4-({(2S)-2-[2-(4-chlorophenyl)-5,6-difluoro-1H-benzimidazol-1-yl]-2-cyclohexylacetyl}amino)-3,5-difluorobenzoic acid | C28 H22 Cl F4 N3 O3 | 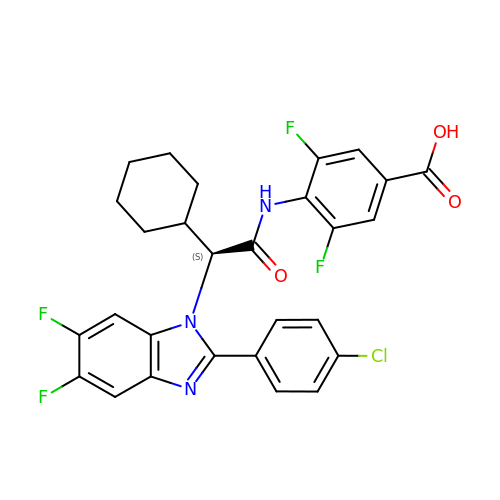MRVUTCGFXDGVGC-VWLOTQADSA-N>GMSQPKKRKLESGGGGEGGEGTEEEDGAEREAALERPRRTKRERDQLYYECYSDVSVHEEMIADRVRTDAYRLGILRNWAALRGKTVLDVGAGT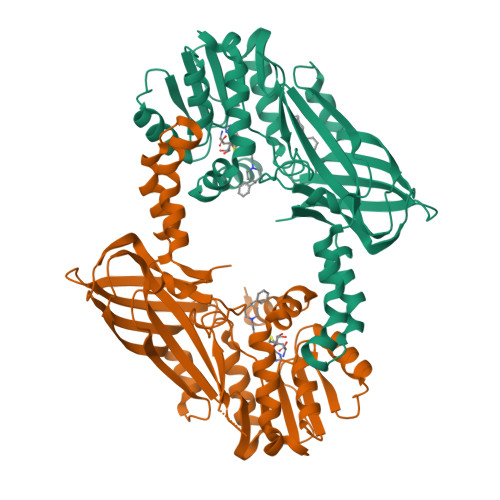GILSIFCAQAGARRVYAVEASAIWQQAREVVRFNGLEDRVHVLPGPVETVELPEQVDAIVSEWMGYGLLHESMLSSVLHARTKWLKEGGLLLPASAELFIVPISDQMLEWRLGFWSQVKQHYGVDMSCLEGFATRCLMGHSEIVVQGLSGEDVLARPQRFAQLELSRAGLEQELEAGVGGRFRCSCYGSAPMHGFAIWFQVTFPGGESEKPLVLSTSPFHPATHWKQALLYLNEPVQVEQDTDVSGEITLLPSRDNPRRLRVLLRYKVGDQEEKTKDFAMED[4x]>GAMAAEMDWDKTVGAAEDVRRIFEHIPAILVGLEGPDHRFVAVNAAYRGFSPLLDTVGQPAREVYPELEGQQIYEMLDRVYQTGEPQSGSEWRLQTDYDGSGVEERYFDFVVTPRRRADGSIEGVQLIVDDVTSRVRARQAAEARVEELSERYRNVRD[4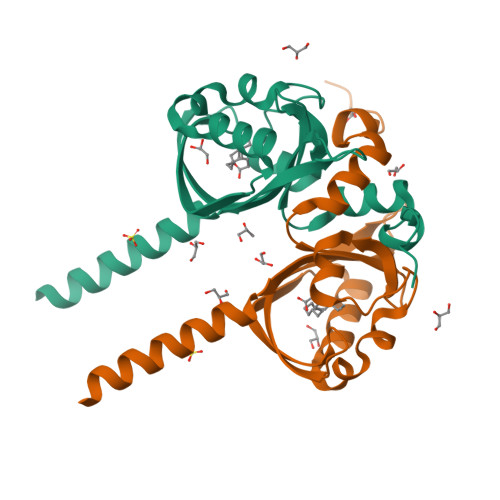x]>GSHMAAGGDHGSPDSYRSPLASRYASPEMCFVFSDRYKFRTWRQLWLWLAEAEQTLGLPITDEQIQEMKSNLENIDFKMAAEEEKRLRHDVMAHVHTFGHCCPKAAGIIHLGATSCYVGDNTDLIILRNALDLLLPKLARVISRLADFAKERASLPTLGFTHFQPAQLTTVGKRCCLWIQDLCMDLQNLKRVRDDLRFRGVKGTTGTQASFLQLFEGDDHKVEQLDKMVTEKAGFKRAFIITGQTYTRKVDIEVLSVLASLGASVHKICTDIRLLANLKEMEEPFEKQQIGSSAMPYKRNPMRSERCCSLARHLMTLVMDPLQTASVQWFERTLDDSANRRICLAEAFLTADTILNTLQNISEGLVVYPKVIERRIRQELPFMATENIIMAMVKAGGSRQDCHEKIRVLSQQAASVVKQEGGDNDLIERIQADAYFSPIHSQLDHLLDPSSFTGRASQQVQRFLEEEVYPLLKP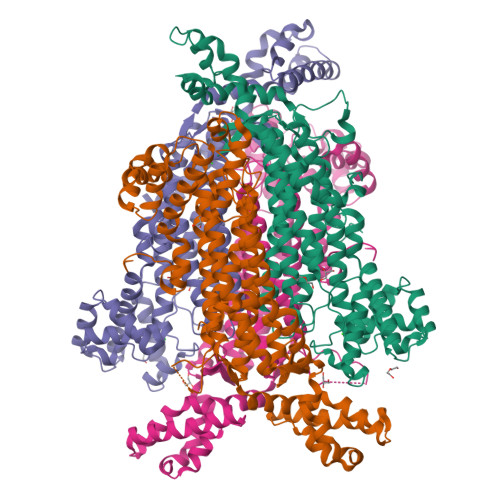YESVMKVKAELCL[4x]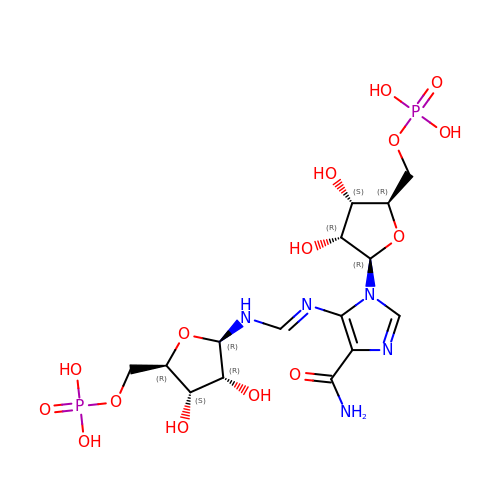[(2R,3S,4R,5R)-5-[4-aminocarbonyl-5-[(E)-[[(2R,3R,4S,5R)-3,4-bis(oxidanyl)-5-(phosphonooxymethyl)oxolan-2-yl]amino]methylideneamino]imidazol-1-yl]-3,4-bis(oxidanyl)oxolan-2-yl]methyl dihydrogen phosphate | C15 H25 N5 O15 P2 | QOUSHGMTBIIAHR-KEOHHSTQSA-N>[2x]TPEMPVLENRAAQGNITAPGGARRLTGDQTAALRNSLSDKPAKNIILLIGDGMGDSEITAARNYAEGAGGFFKGIDALPLTGQYTHYALNKKTGKPDYVTDSAASATAWSTGVKTYNGALGVDIHEKDHPTILEMAKAAGLATGNVSTAELQGATPAALVAHVTSRKCYGPSKTSQKCPGNALEKGGKGS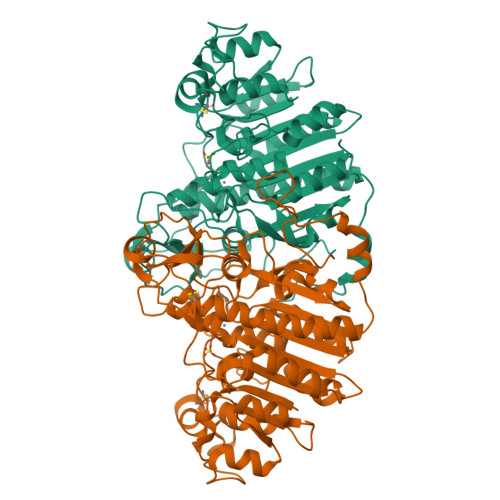ITEQLLNARADVTLGGGAKTFAETATAGEWQGKTLREEAEARGYQLVSDAASLNSVTEANQQKPLLGLFADGNMPVRWLGPKATYHGNIDKPAVTCTPNPQRNDSVPTLAQMTDKAIELLSKNEKGFFLQVEGASIDKQNHAANPCGQIGETVDLDEAVQRALEFAKKEGNTLVIVTADHAHASQIVAPDTKAPGLTQALNTKDGAVMVMSYGNSEEDSQEHTGSQLRIAAYGPHAANVVGLTDQTDLFYTMKAALGLK4-O-(4-O-SULFONYL-N-ACETYLGLUCOSAMININYL)-5-METHYLHYDROXY-L-PROLINE-TAURINE | C16 H30 N3 O14 S2 | 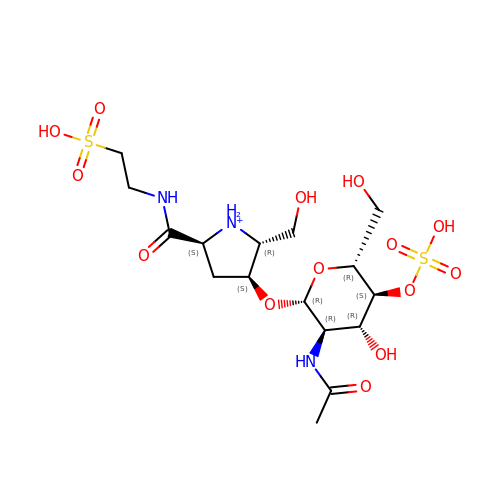RPNZWZDLNYCCIG-HMMVDTEZSA-O> ALESAQESHALHHQNAAALRFQFHITREQAREIVKLCPNCPDWGHAPQLGVNPRGLKPRVLWQMDVTHVSEFGKLKYVHVTVDTYSHFTFATARTGEATKDVLQHLAQSFAYMGIPQKIKTDNAPAYVSRSIQEFLARWKISHVTGIPYNPQGQAIVERTHQNIKAQLNKLQKAGKYYTPHHLLAHALFVLN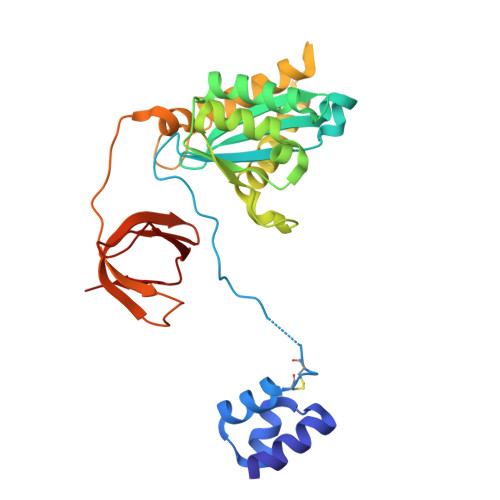HVNMDNQGHTAAERHWGPISADPKPMVMWKDLLTGSWKGPDVLITAGRGYACVFPQDAESPIWVPDRFIRPFT>MQSDTQE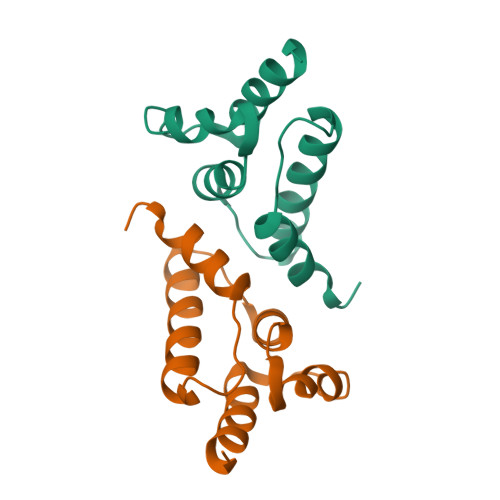ANDIVTLVNLQYNGSTPADAFETKVTNIIDRLNNNGIHINNKVACQLIMRGLSGEYKFLRYTRHRHLNMTVAELFLDIHAIYEEQQGSRNPLEHHHHHH[3x]> GSHMRNVAAEQQLRELESTFDGRLGFVALDTATGARIAHRADERFPFYSTFKTMLSAAVLARSAGDAALLQRRIPYAKRDLVR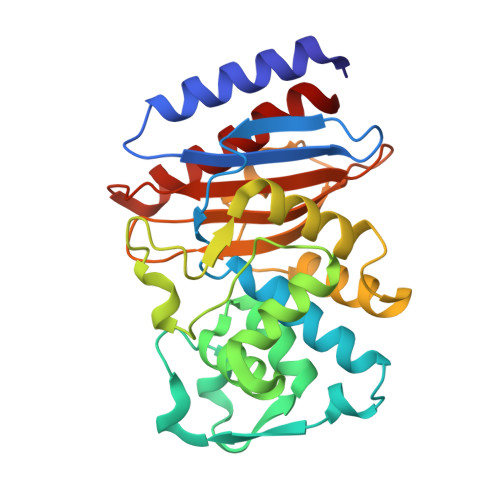YSPITEKHVGAGMTVAELCAATLQYSDNTAANLLIALLGGPQAVTAYARSIGDATFRLDRRETELNTAIPGDERDTTTPAAMAASVRRLLVGDALGTAQRAQLNAWMLGNKTGDARIRAGVPAGWRVADKTGTGDYGTGNDIGVAYPPDRAPIVFVVYTTMRSRNAQARDDVIASAARIAARAFV> 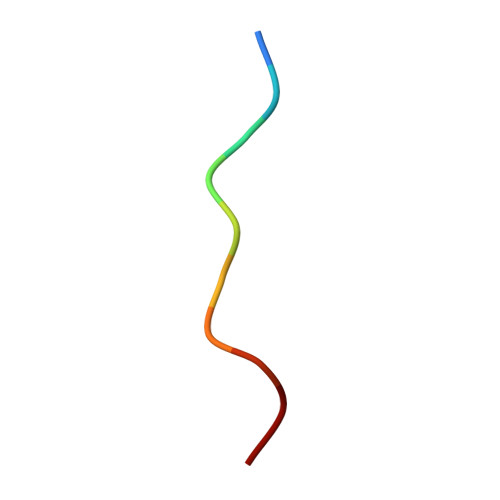VPPPVPPPPS> FHLGKCPNPPVQENFDVNKYPGRWYEIEKIPTTFENGRCIQANYSLMENGKIKVLNQELRADGTVNQIEGEATPVNLTEPAKLEVKFSWFMPSAPYHILATDYENYALVYSCTSISQSFHVD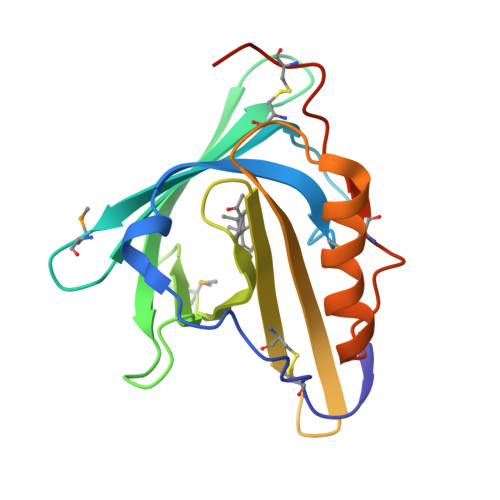FAWILARNVALPPETVDSLKNILTSNNIDVKKMTVTDQVNCPKLSAHHHHHH> GELELHPPAFPWSHGGPLSALDHSSVRRGFQVYKQVCSACHSMDYVAFRNLIGVTHTEAEAKALAEEVEVQDGPDENGELFMRPGKISDYFPKPYPNPEAARAANNGALPPDLSYIVNARHGGEDYVFSLLTGYCDPPAGVVVREGLHYNPYFPGQAIGMAPPIYNEILEYDDGTPATMSQIAKDVCTFLRWAAEPEHDQRKRMGLKMLLISALLTSLLYYMKRH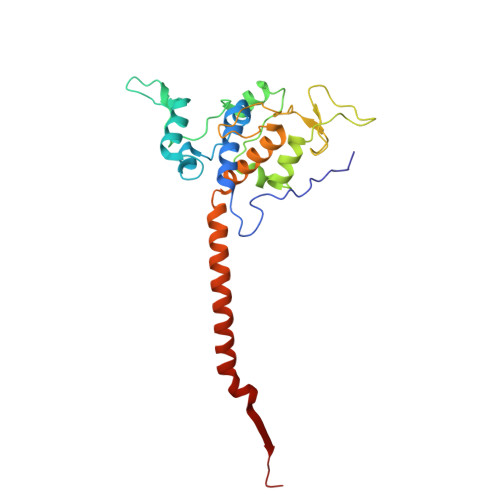KWSVLKSRKMAYRPPK(1S,2S,3S,4R,5R)-2-[(furan-2-ylmethyl)amino]-4-(piperidin-1-yl)-6,8-dioxabicyclo[3.2.1]octan-3-ol 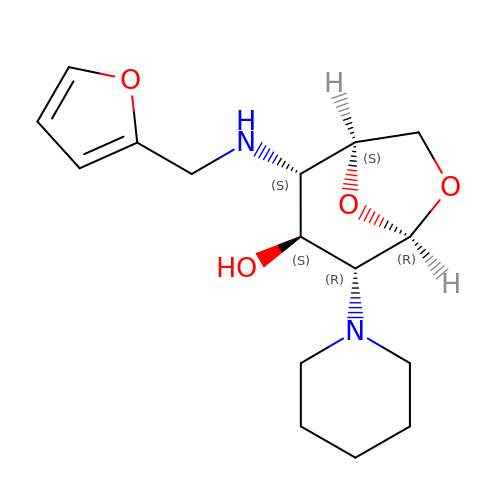| C16 H24 N2 O4 | UGNVVIUBNSMYSH-DGXTUMSLSA-N> XXXXXXXXXXXXXXXXXXXXXAYDAQVKNDEQDVELAD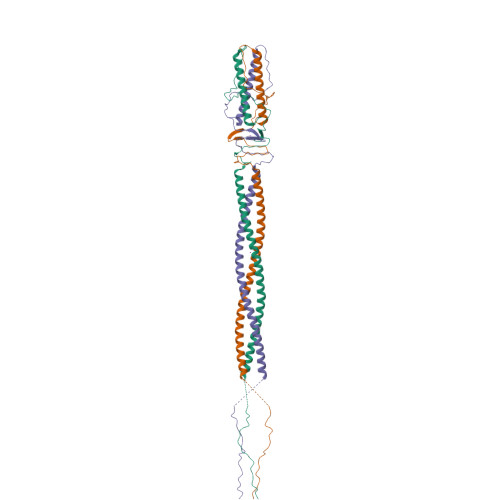HDARIAANTKAINILEVRLTTAEGKIVVLRSDVDYLLDEVIDIQAHLVTVDQRLDGVESDVSDIKSDYVSKTVTESQSLASPLDVKTSYSVDGIQVVGARQTGWTAATGTPLLGSFNANQSYTVGTTYTQSEVAALATGLEQARQRILALETALRLHGLID;> MADSNLNEPVIIQATRLDTSILPRNIFSQSYLLYVIAQGTDVGNVANKANEAGQGAYDAQVKNDEQDVELADHDARIAANTKAINILEVRLTTAEGKIVVLRSDVDYLLDEVIDIQAHLVTVDQRLDGVESDVSDIKSDYVSKTVTESQSLASPLDVKTSYSVDGIQVVGARQTGWTAATGTPLLGSFNANQSYTVGTTYTQSEVAALATGLEQARQRILALETALRLHGLID>[2x]QIMEPHDTLSPAQVDEYRKNGFLVQEHVFDEEEIELLRAEAAQEFASGGERVTVEQNTGIVRGVHGCHLYSEVFGRLVRSPRLLPIARQLLRDDVYVHQFKINAKRAFKGEVWEWHQDYTFWHHEDGMPAPRALSAA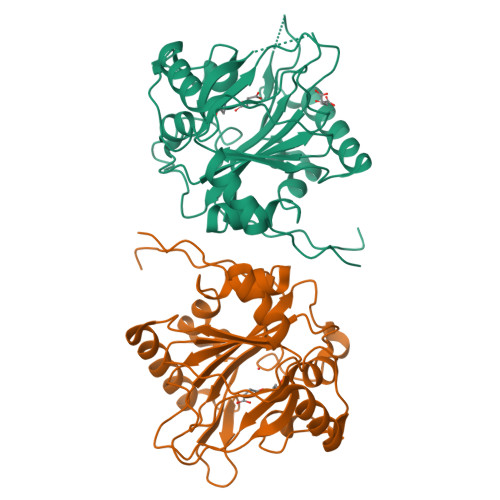IFLDEVTEFNGPLTFVPGGHGSGMIDADVKGEGWANTLTASLKYSLDVETMRGLIERNGMVAPKGPRGSVLWFDANIPHSSVPNISPFDRGLVLITYNSVENKTDVTRGTRPEWLAARDFTPLTALQATSF PfRh5 is a member of the PfRh family and binds specifically to the receptor basigin on the human erythrocyte surface. This protein plays an essential role in merozoite invasion and host tropism of P. falciparum. It forms a complex with the cysteine-rich protein PfRipr during merozoite invasion; the complex is peripherally associated with parasite membranes and is released at the apical end of the merozoite during invasion of the human erythrocyte. Antibodies to PfRh5 can block merozoite invasion, suggesting that it is a potential vaccine candidate.

We determined the N-terminal amino acid sequence by mass spectrometry and re-expressed this region in insect cells to produce a highly stable module of PfRh5 that we denote PfRh5-C. The shape of PfRh5-C approximates an elliptical disk, the core consisting of nine mostly anti-parallel α-helices that encase a small β-hairpin located near the N-terminus. Helices α4, α5, α6, and α7 assemble as a triplet-helical coiled-coil domain running the length of the long axis of the molecule. On the opposite side to the α4/α5/α6/α7 coiled-coil domain, helices α1, α2a, and α3b assemble to form a short three-helix bundle and helices α2b and α3a assemble to form a short two-helix coiled-coil domain, these domains being approximately half the length of the α4/α5/α6/α7 coiled-coil domain. The first disulphide bond is Cys345–Cys351, located at one apex of the helical bundle. The second disulphide bond is Cys224–Cys317; Cys224 lies close to the N-terminus of helix α2b and Cys317 close to the C-terminus of helix α3a, that is, in proximity to ‘kink points’ of the parent helices α2 and α3. Electron density for residues 258–293 is absent, indicating partial disorder of this loop within the crystal structure. A search using DALI indicates that the PfRh5 fold is novel. Comparison of the Rh5 structure in the bound and unbound state shows that there are no changes in the core structure on binding of receptor.

> GTDVKNNEDYKNVDYKNVNFLQYHFKELSNYNIANSIDILQEKEGHLDFVIIPHYTFLDYYKHLSYNSIYHKSSTYGKCIAVDAFIKKINETYDKVKSKCNDIKNDLIATIKKLEHPYDINNKNDDSYRYDISEEIDDKSEETDDETEEVEDSIQDTDSNHTPSNKKKNDLMNRTFKKMMDEYNTKKKKLIKCIKNHENDFNKICMDMKNYGTNLFEQLSCYNNNFCNTNGIRYHYDEYIHKLILSVKSKNLNKDLSDMTNILQQSELLLTNLNKKMGSYIYIDTIKFIHKEMKHIFNRIEYHTKIINDKTKIIQDKIKLNIWRTFQKDELLKRILDMSNEYSLFITSDHLRQMLYNTFYSKEKHLNNIFHHLIYVLQMKFNDVPIKMEYFQTYKKNKPLTQ> MSRNGELCLQRIIVSYSPNKGNPAMRQFMATHLPEFHRQYPQVKIDIRPRQWPESSITGIYRDGSEKA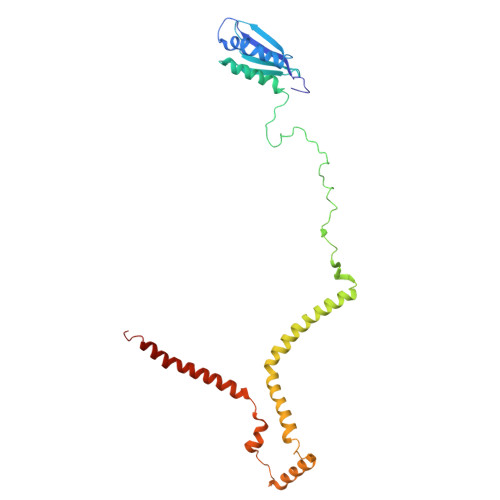YSIRFLSSMGINVRFHRLVNEGNDYNHSFSASHLHLQRRSVQGTWNPYLWNYEGTRARHKPPAQWSRKLTEKEWDYYVQQYGAQMKAEEDTIADRVRRYTDIPEASTEEVNQRWKEHVMPRLQTDLEYNLSHWKKQHRTGAGRPAPPTLNEYSLFSVPDHSSLGQDAIDMLRRREAQREEDWWRERKGQLKPPE2,5-DIOXOPENTANOIC ACID | C5 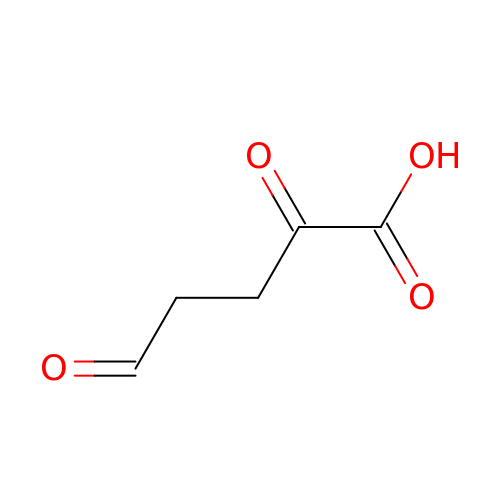H6 O4 | VHKNBDIQDAXGBL-UHFFFAOYSA-N>SNAMTETQSLELAKELISRPSVTPDDRDCQKLLAERLHKIGFAAEELHFGDTKNIWLRRGTKAPVVCFAGHTDVVPTGPVEKWDSPPFEPAERDGRLYGRGAADMKTSIACFVTACERFVAKHPNHQGSIALLITSDEEGDALDGTTKVVDVLKARDELIDYCIVGEPTAVDKLGDMIKNGRRGSLSGNL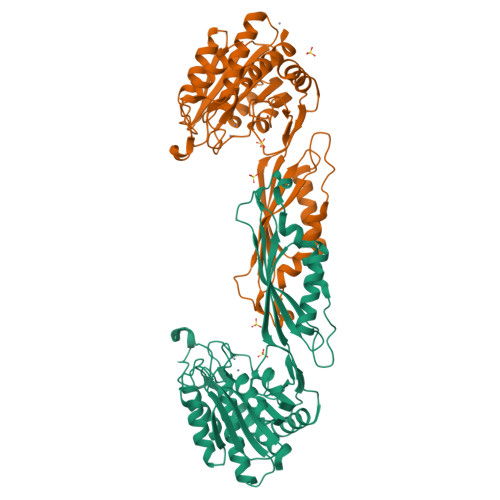TVKGKQGHIAYPHLAINPVHTFAPALLELTQEVWDEGNEYFPPTSFQISNINGGTGATNVIPGELNVKFNFRFSTESTEAGLKQRVHAILDKHGVQYDLQWSCSGQPFLTQAGKLTDVARAAIAETCGIEAELSTTGGTSDGRFIKAIAQELIELGPSNATIHQINENVRLNDIPKLSAVYEGILARLLAGNAV[2x]> SMPDGYLKLPDDWVRVMVSVPAPVDEVWEAVTDPRRVAQWFGHLSAPMTTGASTRVDFGDGDFFDIEVDHVEPRDRLLFRWSFLGVGPECQVGWTLT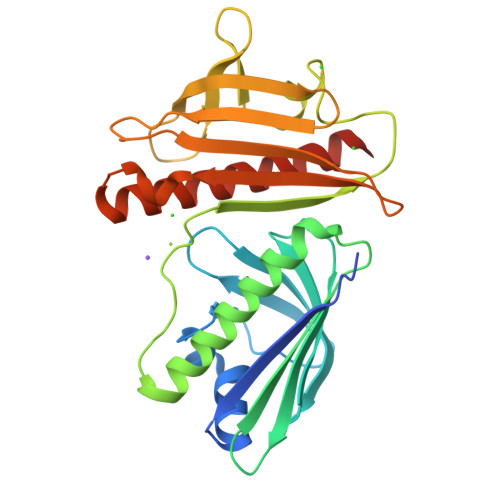GGAEATTLTVDDSCPGRPGSEVAQLKAGWLDFVGRLARYLETGKPSRYDWRQEIDGSVVLPNGSWHPLREETVVDWLPIATNGAGPGWFFVVDEEGPRRFTLRDWQLDRERALTFAVEIPGARTVTACQVRTEPGERGRTLSVSHQGWHRLGLSDLQERTLRHRFAATWTAALSLAEECARTRQELP>[2x]EMCEIPEMDSHLVEKLGQHLLPWMDRLSLEHLNPSIYVGLRLSSLQAGTKEDLYLHSLKLGYQQCLLGSAFSEDDGDCQGKPSMGQLALYLLALRANCEFVRGHKGDRLVSQLKWFLEDEKRAIGHDHKGHPHTSYYQYGLGILALCLHQKRVHDSVVDKLLYAVEPFHQGHHSVDTAAMAGLAFTCLKRSNFNPGRRQRITMAIRTVQEEILKAQTPEGHFGNVYSTPLALQFLMTSPMRGAELGTACLKARVALLASLQDGAFQNALMISQLLPVLNHKTYIDLIFPDCLAPRVMLEPAAETIPQTQEIISVTLQVLSLLPPYRQSISVLAGSTVEDVLKKAHELGGFTYETQASLSGPYLTSVMGKAAGEREFWQLLRDPNTPLLQGIADYRPKDGETIELRLVSW;>[2x]SCPPTKFQCRTSGLCVPLTWRCDRDLDCSDGSDEEECRIEPCTQKGQCPPPPGLPCPCTGV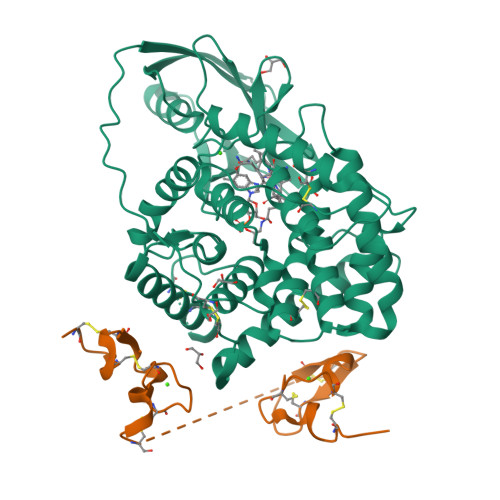SDCSGGTDKKLRNCSRLACLAGELRCTLSDDCIPLTWRCDGHPDCPDSSDELGCGTNE>MKKRLAYAIIQFLHDQLRHGGLSSDAQESLEVAIQC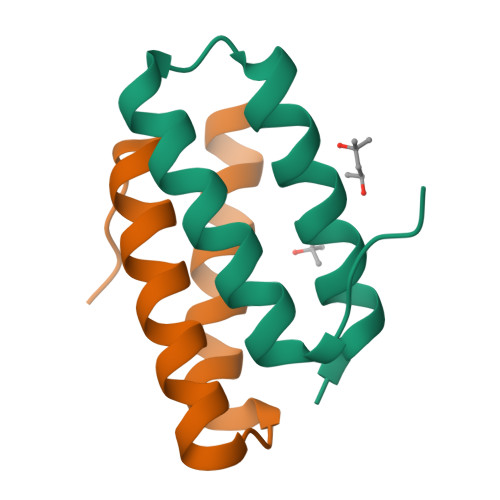LETAFGVTVEDSDLAL[2x]> MNITSLQQNITRSWQIPFTNSSDSIVTVGDRNLTIDEVVNVARHGTQVRLTDNADVIRGVQASCDYINNAVETAQPIYGVTSGFGGMADVVISREQAAELQTNLIWFLKSGAGNKLSLADVRAAMLLRANSHLYGASGIRLELIQRIETFLNAGVTPHVYEFGSIGASGDLVPLSYITGALIGLDPSFTVDFDGKEMDAVTALSRLGLPKLQLQPKEGLAMMNGTSVMTGIAANCVYDAKVLLALTMGVHALAIQGLYGTNQS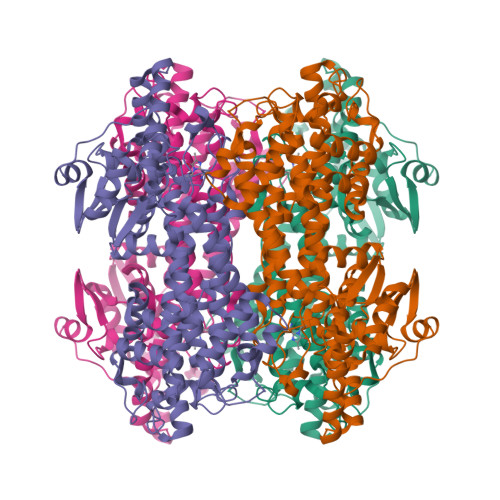FHPFIHQCKPHPGQLWTADQMFSLLKDSSLVREELDGKHEYRGKDLIQDRYSLRCLAQFIGPIVDGVSEITKQIEVEMNSVTDNPLIDVENQVSYHGGNFLGQYVGVTMDRLRYYIGLLAKHIDVQIALLVSPEFSNGLPPSLVGNSDRKVNMGLKGLQISGNSIMPLLSFYGNSLADRFPTHAEQFNQNINSQGYISANLTRRSVDIFQNYMAIALMFGVQAVDLRTYKMKGHYDARTCLSPNTVQLYTAVCEVVGKPLTSVRPYIWNDNEQCLDEHIARISADIAGGGLIVQAVEHIFSSLKST>GMKTSVKFETIFPLTTAPLIQCITNEITCESMANALLYIDAKPIMADDPREFPQMFQQTSALVLNLGHLSQEREQSLLAASDYARQVNKLTVVDLVGYGASDIRNEVGEKLVHNQPTVVKGNLSEMR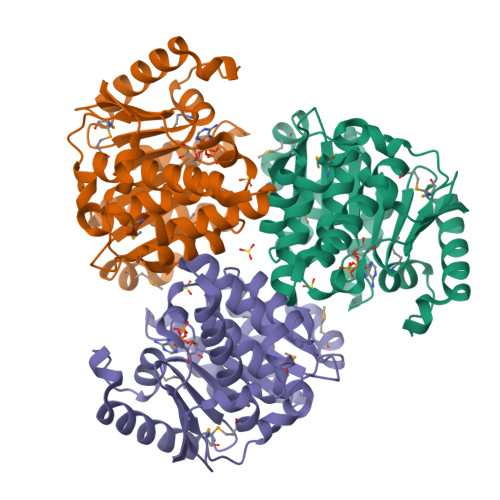TFCQLVSHGRGVDGSPLDQSEEAIEELIQALRQQTQKFPQTVFLATGIQDVLVSQEQVIVLQNGVPELDCFTGTGDLVGALVAALLGEGNAPMTAAVAAVSYFNLCGEKAKTKSQGLADFRQNTLNQLSLLMKEKDWFEAVKGRVL[2x]> WSHPQFEKSGMAVDTGTEVVYRRPEARDGTRVWELIRDTGSLDLNSPYCYMLLG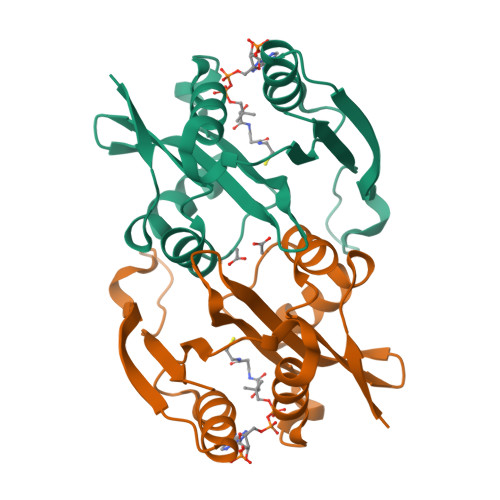DYFNDTCMIAEHEGDIVGFISAFRSPRNPETLFVWQVAVASSHRRQGIAKAMLTGLMNQKACHGVRFIETTVSPSNMASRRLFLGYAEEKSIPSTVTVGYGAEMFPDGTTHEDEPLFVIGPFFNDIGSAWSH> GAMGSFNSIDVEINMYPVNKTSCNSSIGSSSTISTSELTITLTHEDCTPVFIGDYYSVVDKLATSGFFTNDKVHQDLTTQCKINLEIKCNSGRESRQLTPTTKVYLMPHSETVTVVGDCLSNLDVYIVYANTDAIYSDMDVVA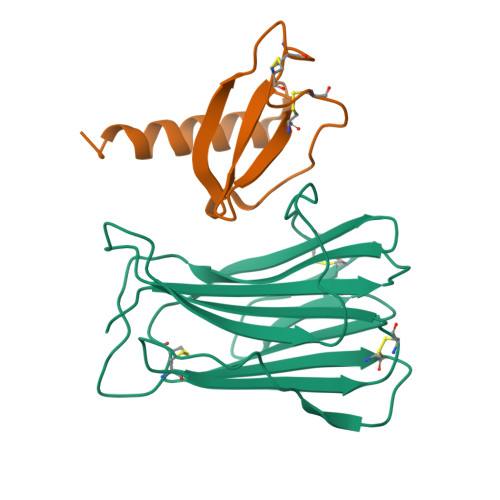YHTSYILNVDHIPPNDCERD;> GAMGQHHGVTKCNITCSKMTSKIPVALLIHYQQNQASCGKRAIILETRQHRLFCADPKEQWVKDAMQHLDRQAAALTRNG>GYITVGNENSTPIELYYEDQGSGQPVVLIHGYPLDGHSWERQTRELLAQGYRVITYDRRGFGGSSKVNTGYDYDTFAADLHTVLETLDLRDVVLVGFSMGTGELARYVARYGHERVAKLAFLASLEPFLVQRDDNPEGVPQEVFDGIEAAAKGDRFAWFTDFYKNFYNLDENLGSRI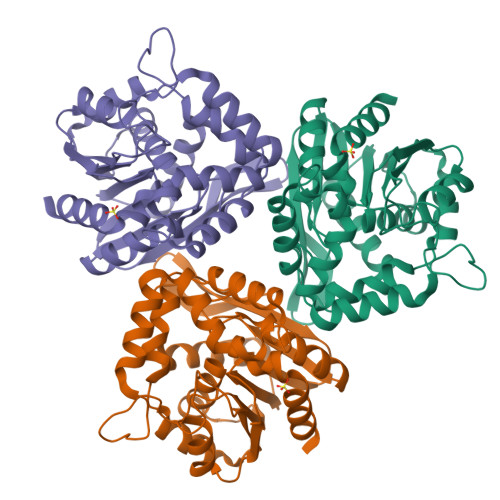SEQAVTGSWNVAIGSAPVAAYAVVPAWIEDFRSDVEAVRAAGKPTLILHGTKDNILPIDATARRFHQAVPEADYVEVEGAPHGLLWTHADEVNAALKTFLAK[2x]> MEIPVIEPLFTKVTEDIPGAEGPVFDKNGDFYIVAPEVEVNGKPAGEILRIDLKTGKKTVICKPEVNGYGGIPAGCQCDRDANQLFVADMRLGLLVVQTDGTFEEIAKKDSEGRRMQGCNDCAFDYEGNLWITAPAGEVAPADYTRSMQEKFGSIYCFTTDGQMIQVDTAFQFPNGIAVRHMNDGRPYQLIV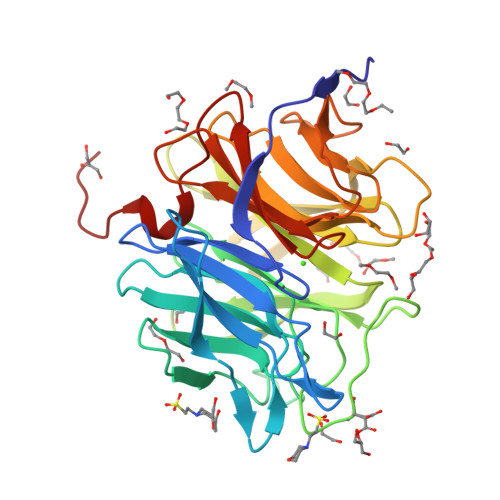AETPTKKLWSYDIKGPAKIENKKVWGHIPGTHEGGADGMDFDEDNNLLVANWGSSHIEVFGPDGGQPKMRIRCPFEKPSNLHFKPQTKTIFVTEHENNAVWKFEWQRNGKKQYCETLKFGIF> MITTPLVHVASVEKGRSYEDFQKVYNAIALKLR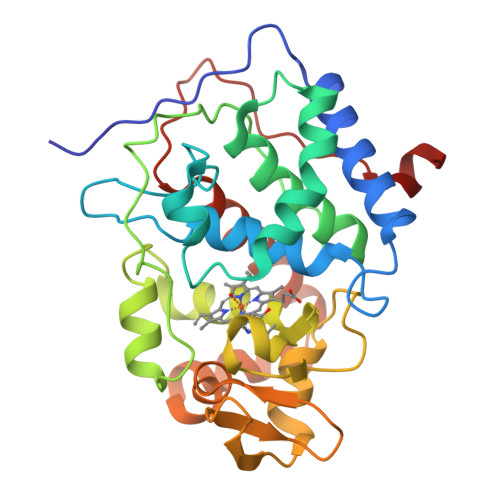EDDEYDNYIGYGPVLVRLAWHISGTWDKHDNTGGSYGGTYRFKKEFNDPSNAGLQNGFKFLEPIHKEFPWISSGDLFSLGGVTAVQEMQGPKIPWRCGRVDTPEDTTPDNGRLPDADKDAGYVRTFFQRLNMNDREVVALMGAHALGKTHLKNSGYEGPWGAANNVFTNEFYLNLLNEDWKLEKNDANNEQWDSKSGYMMLPTDYSLIQDPKYLSIVKEYANDQDKFFKDFSKAFEKLLENGITFPKDAPSPFIFKTLEEQGL~{N}-methyl-1-(3-thiophen-3-ylphenyl)methanamine | C12 H13 N S | 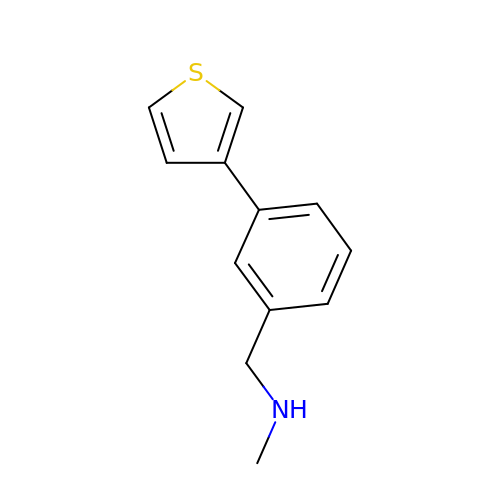SNXSVYZFYWVLHK-UHFFFAOYSA-N MRV is a prototypical member of the Reoviridae family of segmented double-stranded RNA (dsRNA) viruses, which is further divided into two subfamilies based on the presence or absence of turrets on the inner capsids: turreted (Spinareovirinae, including MRV) and nonturreted (Sedoreovirinae, including bluetongue virus (BTV) and the life-threatening rotavirus). MRV capsids are composed of two concentric protein layers, encapsulating 10 dsRNA segments. The outer layer of MRV consists of the protection protein σ3, membrane penetration protein μ1, and spike protein σ1. The inner layer consists of proteins λ1, σ2, and turret protein λ223.

Inside the particle, reconstructions of virion and core particles clearly show that the layered RNA genome and densities of TEC (at red arrows) are underneath the inner shell, indicating that genome replication from ssRNA to dsRNA has been completed in the core. All genome-filled core particles have the turret attached at the fivefold axis. Thus, RNA genome may facilitate turret attachment. Five λ2 subunits form a pentameric turret at each of the fivefold axes, serving as the mRNA exit channel. The λ2 pentameric turret changes conformation during virus assembly: in the core, the turret is open, with a central channel 75 Å in diameter; in the virion, it closes, sealing off the channel. In the open conformation, the Ig-like domains of λ2 straighten, forming the channel for mRNA capping and export. Unlike the core observed in this study with an open turret, the crystal structure of the MRV core, which was obtained on samples generated from chymotrypsin-digested virions, shows the turret in the same closed conformation as that in the virion. Studies have shown that assembled core particles in the condensates are active in mRNA transcription, but this activity is inhibited after outer layer proteins μ1/σ3 and σ1 are incorporated to form virion particles. Our structural data align with these functional findings: in the core, the open conformation of the turret maximally facilitates mRNA export efficiency, while in the virion, the closed conformation of the turret suppresses transcription, leading to a virion in the quiescent state. Due to the limited number of particles, we were unable to obtain an asymmetric reconstruction of the core with TEC resolved inside.

> ANVWGVRLADSLSSPTIETRTRQYTLHDLCSDLDANPGREPWKPLRNQRTNNIVAVQLFRPLQGLVLDTQLYGFPGAFDDWERFMREKLRVLKYEVLRIYPISNYSNEHVNVFVANALVGAFLSNQAFYDLLPLLIINDTMIGDLLGTGASLSQFFQSHGDVLEVAAGRKYLQMENYSNDDDDPPLFAKDLSDYAKAFYSDTYEVLDRFFWTHDSSAGVLVHYDKPTNGHHYLLGTLTQMVSAPPYIINATDAMLLESCLEQFSANVRARPAQPVTRLDQCYHLRWGAQYVGEDSLTYRLGVLSLLATNGYQLARPIPRQLTNRWLSSFVSQIMSDGVNETPLWPQERYVQIAYDSPSVVDGATQYGYVRKNQLRLGMRISALQSLSDTPSPVQWLPQYTIDQAAMDEGDLMVSRLTQLPLRPDYGNIWVGDALSYYVDYNRSHRVVLSSELPQLPDTYFDGDEQYGRSLFSLARKIGDRSLVKDTAVLKHAYQAIDPNTGKEYLRSRQSVAYFGASAGHSGADQPLVIEPWIQGKISGVPPPSSVRQFGYDVARGAIVDLARPFPSGDYQFVYSDVDQVVDGHDDLSISSGLVESLLSSCMHATAPGGSFVVKINFPTRPVWHYIEQKILPNITSYMLIKPFVTNNVELFFVAFGVHQHSSLTWTSGVYFFLVDHFYRYETLSTISRQLPSFGYVDDGSSVTGIETISIENPGFSNMTQAARIGISGLCANVGNARKSIAIYESHGARVLTITSRRSPASARRKSRLRYLPLIDPRSLEVQARTILPADPVLFENVSGASPHVCLTMMYNFEVSSAVYDGDVVLDLGTGPEAKILELIPATSPVTCVDIRPTAQPSGCWNVRTTFLELDYLSDGWITGVRGDIVTCMLSLGAAAAGKSMTFDAAFQQLIKVLSKSTANVVLVQVNCPTDVVRSIKGYLEIDSTNKRYRFPKFGRDEPYSDMDALEKICRTAWPNCSITWVPLSYDLRWTRLALLESTTLSSASIRIAELMYKYMPIMRIDIHGLPMEKRGNFIVGQNCSLVIPGFNAQDVFNCYFNSALAFSTEDVNAAMIPQVSAQFDATKGEWTLDMVFSDAGIYTMQALVGSNANPVSLGSFVVDSPDVDITDAWPAQLDFTIAGTDVDITVNPYYRLMTFVRIDGQWQIANPDKFQFFSSASGTLVMNVKLDIADKYLLYYIRDVQSRDVGFYIQHPLQLLNTITLPTNEDLFLSAPDMREWAVKESGNTICILNSQGFVLPQDWDVLTDTISWSPSIPTYIVPPGDYTLTPL;>[3x]MKRIPRKTKGKSSGKGNDSTERADDGSSQLRDKQNNKAGPATTEPGTSNREQYKARPGIASVQRATESAEMPMKNNDEGTPDKKGNTKGDLVNEHSEAKDEADEATKKQAKDTDKSKAQVTYSDTGINNANELSRSGNVDNEGGSNQKPMSTRIAEATSAIVSKHPARVGLPPTASSGHGYQCHVCSAVLFSPLDLDAHVASHGLHGNMTLTSSDIQRHITEFISSWQNHPIVQVSADVENKKTAQLLHADTPRLVTWDAGLCTSFKIVPIVPAQVPQDVLAYTFFTSSYAIQSPFPEAAVSRIVVHTRWASNVDFDRDSSVIMAPPTENNIHLFKQLLNTETLSVRGANPLMFRANVLHMLLEFVLDNLYLNRHTGFSQDHTPFTEGANLRSLPGPDAEKWYSIMYPTRMGTPNVSKICNFVASCVRNRVGRFDRAQMMNGAMSEWVDVFETSDALTVSIRGRWMARLARMNINPTEIEWALTECAQGYVTVTSPYAPSVNRLMPYRISNAERQISQIIRIMNIGNNATVIQPVLQDISVLLQRISPLQIDPTIISNTMSTVSESTTQTLSPASSILGKLRPSNSDFSSFRVALAGWLYNGVVTTVIDDSSYPKDGGSVTSLENLWDFFILALALPLTTDPCAPVKAFMTLANMMVGFETIPMDNQIYTQSRRASAFSTPHTWPRCFMNIQLISPIDAPILRQWAEIIHRYWPNPSQIRYGAPNVFGSANLFTPPEVLLLPIDHQPANVTTPTLDFTNELTNWRARVCELMKNLVDNQRYQPGWTQSLVSSMRGTLDKLKLIKSMTPMYLQQLAPVELAVIAPMLPFPPFQVPYVRLDRDRVPTMVGVTRQSRDTITQPALSLSTTNTTVGVPLALDARAITVALLSGKYPPDLVTNVWYADAIYPMYADTEVFSNLQRDMITCEAVQTLVTLVAQISETQYPVDRYLDWIPSLRASAATAATFAEWVNTSMKTAFDLSDMLLEPLLSGDPRMTQLAIQYQQYNGRTFNIIPEMPGSVIADCVQLTAEVFNHEYNLFGIARGDIIIGRVQSTHLWSPLAPPPDLVFDRDTPGVHIFGRDCRISFGMNGAAPMIRDETGLMVPFEGNWIFPLALWQMNTRYFNQQFDAWIKTGELRIRIEMGAYPYMLHYYDPRQYANAWNLTSAWLEEITPTSIPSVPFMVPISSDHDISSAPAVQYIISTEYNDRSLFCTNSSSPQTIAGPDKHIPVERYNILTNPDAPPTQIQLPEVVDLYNVVTRYAYETPPITAVVMGVP;>ARAAFLFKTVGFGGLQNVPINDELSSHLLRAGNSPWQLTQFLDWISLGRGLATSALVPTAGSRYYQMSCLLSGTLQIPFRPNHRWGDIRFLRLVWSAPTLDGLVVAPPQVLAQPALQAQADRVYDCDDYPFLARDPRFKHRVYQQLSAVTLLNLTGFGPISYVRVDEDMWSGDVNQLLMNYFGHTFAEIAYTLCQASANRPWEYDGTYARMTQIVLSLFWLSYVGVIHQQNTYRTFYFQCNRRGDAAEVWILSCSLNHSAQIRPGNRSLFVMPTSPDWNMDVNLILSSTLTGCLCSGSQLPLIDNNSVPAVSRNIHGWTGRAGNQLHGFQVRRMVTEFCDRLRRDGVMTQAQQNQVEALADQTQQFKRDKLETWAREDDQYNQAHPNSTMFRTKPFTNAQWGRGNTGATSAAIAALI[2x]> GSHMVPAALPQLTPTLVSLLEVIEPEVLYAGYDSSVPDSAWRIMTTLNMLGGRQVIAAVKWAKAIPGFRNLHLDDQMTLLQYSWMFLMVFALGWRSYRQASGNLLCFAPDLIINEQRMTLPCMYDQCKHMLFISTELQRLQVSYEEYLCMKTLLLLSSVPKEGLKSQELFDEIRMTYIKELGKAIAKRGGNSSQNWQRFYQLTKLLDSMHDVVENLLSYCFQTFLDKSMSIEFPEMLAE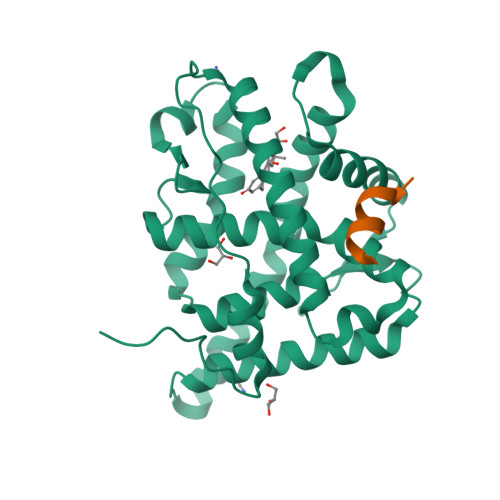IITNQIPKYSNGNIKKLLFHQK;> KENALLRYLLDKD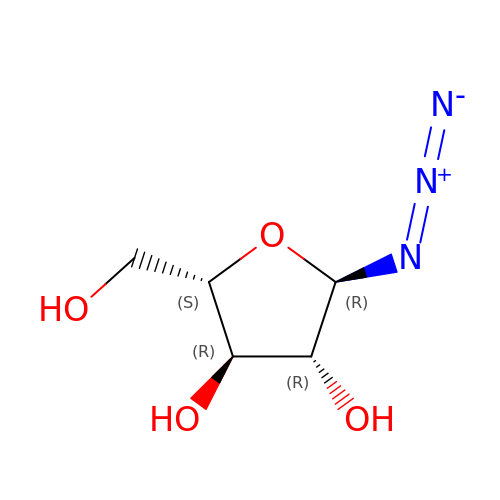(2R,3R,4R,5S)-2-azido-5-(hydroxymethyl)oxolane-3,4-diol | C5 H9 N3 O4 | DHFFHQUOZLQWBU-QMKXCQHVSA-N>[2x]SNAMDYQVPSVALAARVLKLLSRHKYRQSTLTEIAERLGVNKTTCLRVLRTLEREDFVSYDPQSRRYSLGPYLIPLGARAADLNDVYAHALAE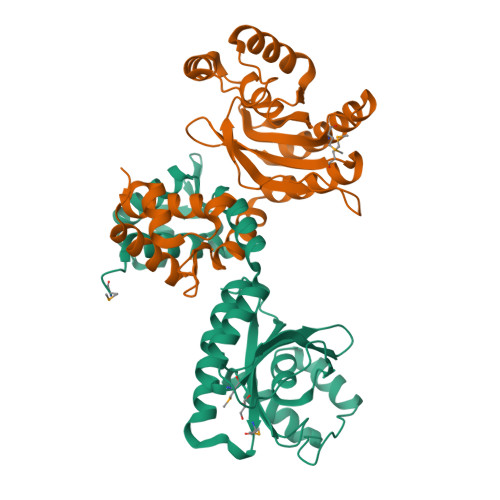LHQVAAHTGMTAVLVKRLRDDRVIYIGSAEPPGDGVRIAVSVGQQFPVYGAAFGRCFLAYDDESTWRRVLREGLKAYTPNSITDEEEYVRLLQEVREKGYAVSHGELWPGISAVAVPVFNQQNKVDLVLSCLTMTSVIQGEDVERAVKALKESAAKVSAWSGYQGRA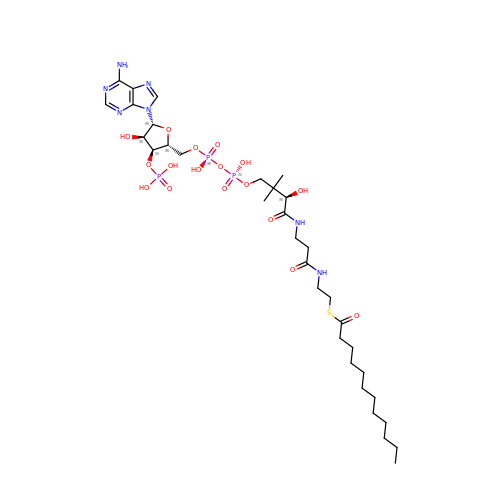DODECYL-COA | C33 H58 N7 O17 P3 S | YMCXGHLSVALICC-GMHMEAMDSA-N Guanosine triphosphate (GTP) cyclohydrolase I (GCH1) (EC:3.5.4.16) catalyzes the conversion of GTP to dihydroneopterin triphosphate (H2NTP). This reaction is the first and rate-limiting step involved in the de novo synthesis of tetrahydrobiopterin (BH4). The effects of GFRP on GCH1 occur via formation of heteromeric protein complexes between GCH1 and GFRP, which are dependent on the intracellular concentrations of the effector molecules phenylalanine or BH4. GCH1−GFRP complexes consist of one GCH1 decamer flanked by two pentameric GFRP complexes.

We determined structures of the human GCH1 in the absence (xtal_GCH1) and presence (xtal_GCH1+active) of the substrate analog 7-deaza-GTP and in the presence of the allosteric inhibitor cpd-1 (xtal_GCH1+allosteric and xtal_GCH1+allosteric). The same degree of disorder seen for the inhibitory cryo-EM structure was observed for the xtal_GCH1_allosteric structure, while region A is ordered and F122 is in a defined closed state in xtal_GCH1+active. The most obvious conformational change upon substrate binding occurs in region A. The partial disorder of the residue range 115 to 130 is resolved into a well-defined loop structure closing the upper ceiling of the active site pocket. This disorder−order transition is clearly seen in both the cryo-EM maps and the X-ray structures. Further, region B involving the triphosphate binding pharmacophore becomes ordered. R216 is part of this region and, in substrate analog complexed states, coordinates the β- and γ-phosphate of GTP variants and contributes to the charge compensation of the triphosphate moiety. Locking the R216 side chain in the presence of triphosphate ligands thus leads to a stabilization of a preferred conformation of this loop. Finally, upon binding of 7-deaza-GTP, changes in region C, including positioning of the five-helix bundle and curvature of the β-barrel, are observed. Here, region C bends outward, toward the active site, and the protein inside expands in comparison to the apo structure. This movement is opposite to the observed conformational change in the inhibitory complex.

>MHHHHHHGSDDDDKRPEAKSAQPADGWKGERPRSEEDNELNLPNLAAAYSSILSSLGENPQRQGLLKTPWRAASAMQFFTKGYQETISDVLNDAIFDEDHDEMVIVKDIDMFSMCEHHLVPFVGKVHIGYLPNKQVLGLSKLARIVEIYSRRLQVQERLTKQIAVAITEALRPAGVGVVVEATHMCMVMRGVQKMNSKTVTSTMLGVFREDPKTREEFLTLIRS[20x]>ALTAKHRPSVVWLHNAECTGCTEAAIRTIKPYIDALILDTISLDYQETIMAAAGEAAEAALHQALEGKDGYYLVVEGGLPTIDGGQWGMVAGHPMIETTKKAAAKAKGIICIGTCSAYGGVQKAKPNPSQAKGVSEALGVKTINIPGCPPNPINFVGAVVHVLTKGIPDLDENGRPKLFYGELVHDNCPRLPHFEASEFAPSFDSEEAKKGFCLYELGCKGPVTYNNCPKVLFNQVNWPVQAGHPCLGCSEPDFWDTMTPFYEQG[3x];>[3x]ASWSHPQFEKGASGAAESKPTPQSTFTGPIVVDPITRIEGHLRIMVEVENGKVKDAWSSSQLFRGLEIILKGRDPRDAQHFTQRACGVCTYVHALASSRCVDDAVKVSIPANARMMRNLVMASQYLHDHLVHFYHLHALDWVDVTAALKADPNKAAKLAASIAPARPGNSAKALKAVQDKLKAFVESGQLGIFTNAYFLGGHKAYYLPPEVDLIATAHYLEALHMQVKAASAMAILGGKNPHTQFTVVGGCSNYQGLTKNPLANYLALSKEVCQFVNECYIPDLLAVAGFYKDWGGIGGTSNYLAFGEFATDDSSPEKHLATSQF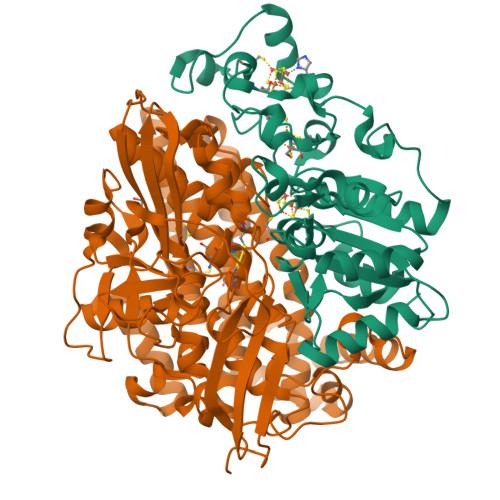PSGVITGRDLGKVDNVDLGAIYEDVKYSWYAPGGDGKHPYDGVTDPKYTKLDDKDHYSWMKAPRYKGKAMEVGPLARTFIAYAKGQPDFKKVVDMVLGKLSVPATALHSTLGRTAARGIETAIVCANMEKWIKEMADSGAKDNTLCAKWEMPEESKGVGLADAPRGALSHWIRIKGKKIDNFQLVVPSTWNLGPRGAQGDKSPVEEALIGTPIADPKRPVEILRTVHAFDPCIACGVH> HMASMKKKGSVVIVGRINLSGDTAYAQQTRGEEGCQETSQTGRDKNQVEGEVQIVSTATQTFLATSINGVLWTVYHGAGTRTIASPKGPVTQMYTNVDKDLVGWQAPQGSRSLTPCTCGSSDLYLVTRHADVIPVRRRGDSRGSLLSPRPISYLKGSSGGPLLCPAGHAVGIFRAAVSTRGVAKAVAFIPVESLETTMRSP

The NS3/4A protease is an excellent target for developing DAAs against HCV, and protease inhibitors have been a key component of most combination therapies. This essential protease cleaves the HCV polyprotein into functional units necessary for viral replication and maturation. Structurally Asp168 is a critical residue that contributes to an active-site electrostatic network necessary for efficient inhibitor binding. We rationally designed HCV protease inhibitors that retain potency while fitting within the substrate envelope to avoid resistance, particularly against D168A, which confers high-level resistance to current HCV PIs.

Increasing the cyclic ring system by one carbon (P4-2) led to a 4-fold increase in potency against the WT. All of the P4 inhibitors were also tested against the D168A RAS and except for P4-2 performed better than the parent compound and grazoprevir (both ∼50 nM), ranging in potency from 2 to 36 nM. The small cyclopropyl ring of P4-1 is able to fit in the S4 pocket better than the larger ring of P4-2. The cyclobutyl ring of P4-2 is actually slightly elevated out of the pocket, similar to the structure of the parent compound, and does not have the conformational flexibility to contour the enzyme. This lack of flexibility results in an unsatisfied or “frustrated” pocket that is neither filled by the inhibitor nor has space for water to easily occupy. Inhibitors with relatively poor potency did not optimally fill the S4 pocket, causing a frustrated pocket that could not be filled by water, a protein side chain, or the inhibitor. This pocket was further destabilized in the D168A variant.>GPLGSVPPTIEQKTRAFTVPNIPLQTLSNSRFPSLIQGMILSPDASQVVQFQNGRCLIDGQLLGTTPATSGQLFRVRGKINQGARTLNLTEVDGKPFMAFDSPAPVGFPDFGKCDWHMRISKTPNNTSSGDPMRSVSVQTNVQGFVPHLGSIQFDEVFNHPTGDYIGTIEWISNPSTPPGTDINLWEIPDYGSSLSQAANLAPPVFPPGFGEALVYFVSAFPGPNNRSAPNDVPCLLPQEYITHFVSEQAPTMGDAALLHYVDPDTNRNLGEFKLYPGGY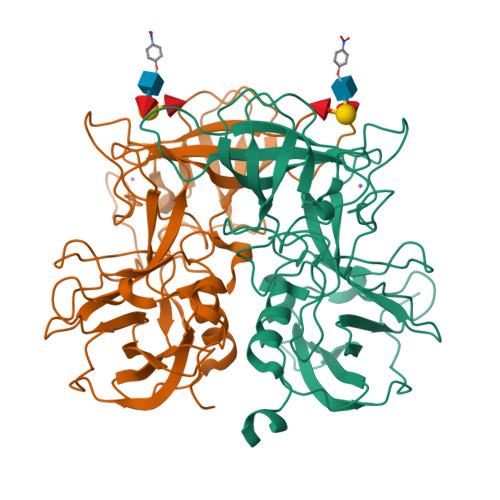LTCVPNGVGAGPQQLPLNGVFLFVSWVSRFYQLKPVGTASTARSRL[2x]>[2x]GPLGRGREEKAPEEPQPVKMPENNSVVEATWNDVQLEDSLGMEVGYRLIPMVDFQQDGELLGRIRSI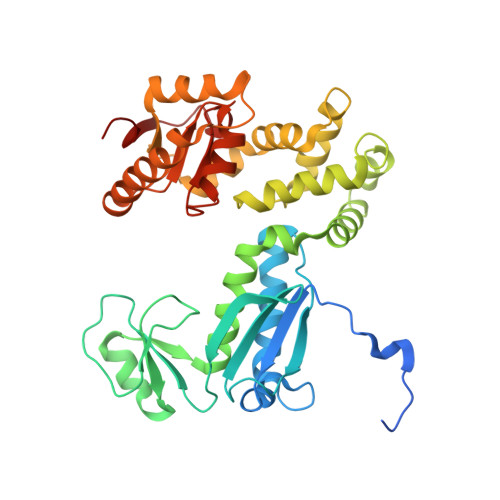RKKFAQDMGFLPPVVHIRDNMDLQPARYRILMKGVEIGSGDAYPGRWLAINPGTAAGTLPGEKTVVPAFGLDAIWIESALKEQAQIQGFTVVEASTVVATHLNHLIGQFSAELFGRQEAQQLLDRVSQEMPKLTEDLVPGVVTLTTLHKVLQNLLAEKVPIRDMRTILETLAEHAPLQSDPHELTAVVRVALGRAITQQWFPGNEEVQVIGLDTALERLLLQALQGGGGLEPGLADRLLAQTQEALSRQEMLGAPPVLLVNHALRPLLSRFLRRSLPQLVVLSNLELSDNRHIRMTATIGGK> MAAALRVAAVGARLSVLASGLRAAVRSLCSQATSVNERIENKRRTALLGGGQRRIDAQHKRGKLTARERISLLLDPGSFVESDMFVEHRCADFGMAADKNKFPGDSVVTGRGRINGRLVYVFSQDFTVFGGSLSGAHAQKICKIMDQAITVGAPVIGLNDSGGARIQEGVESL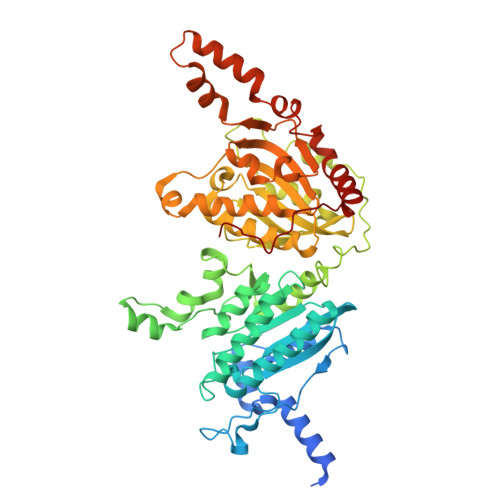AGYADIFLRNVTASGVIPQISLIMGPCAGGAVYSPALTDFTFMVKDTSYLFITGPDVVKSVTNEDVTQEELGGAKTHTTMSGVAHRAFENDVDALCNLRDFFNYLPLSSQDPAPVRECHDPSDRLVPELDTIVPLESTKAYNMVDIIHSVVDEREFFEIMPNYAKNIIVGFARMNGRTVGIVGNQPKVASGCLDINSSVKGARFVRFCDAFNIPLITFVDVPGFLPGTAQEYGGIIRHGAKLLYAFAEATVPKVTVITRKAYGGAYDVMSSKHLCGDTNYAWPTAEIAVMGAKGAVEIIFKGHENVEAAQAEYIEKFANPFPAAVRGFVDDIIQPSSTRARICCDLDVLASKKVQRPWRKHANIPL> DKLGLGREALPEEISAWDTAVLPDGQGLRPGSGDVATGDALFADNCASCHGDFAEGLDSWP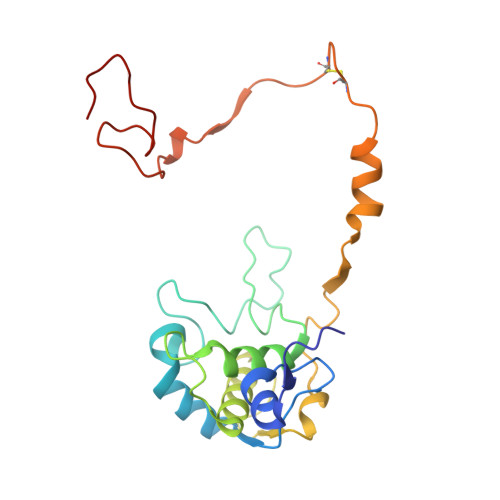VLAGGDGSLTDPRPVKTIGSYWPYLSTVYDYVHRSMPFGSAQTLSVDDTYAITAFLLYSNGLVEDDFVLTHENFTQVVLPNAEGFYPDDRDQTEYPLFSKEPCMTDCAVGVEITKRAVDLNVTPEDPDGRPAGSMPDLGAAAAP> MFFQIEKVVLWSKEAKHKPRVIEFALNKVNLITGSSKSGKSSLIPIIDYCLGSSKCSIPVNTIRDTTAWYGVQIKTKHSRLLIARRDPSNQLSTSNAFFVEAENIEIPQNIEKHNVNIDTVKNRLNEISGVSNISFDFYDTGRIDKKRTSTRDLSAFNYQPQNIIANPNALFYKTDSFEHKSKLVTILPYVLGALSNTDIENQHRIKNLEEEYRKVERRLLKLKRQNEDWLSSAQAYVIKAMELGLVNSDKDIYQLKPERLLNVLKNIATKEIDYSTSAANIKYASEQEAEITKRSRDISNNLAKVKSRLQNINSMNRLANTHSDASRLKRERLSLSKWLLTQNDINSSLFSEPNEIRSLVLEPLARAFSNLEAELEVPIHVQGALSREKIYLEGELTRLASEMKDVNTQLKILRGNKRKLGYDAFSVGKFVGE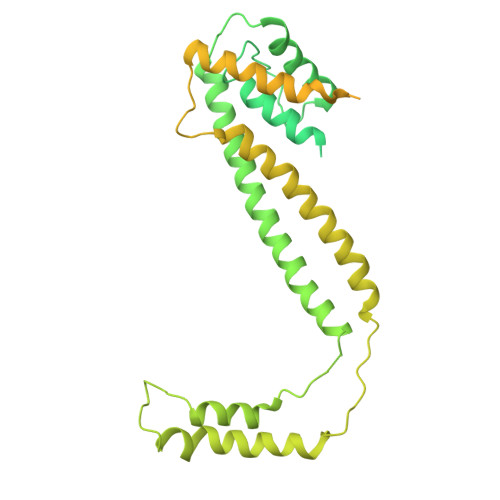VEKALSLMGESESESELSKEYKRLKKELSVLRLKIDPREFERKTKLQLAKVNKLASDWLPHLDTENPNAPISLHEKELTITVNSSGREDYLWEIGSGANWLSYHVAITLALHQHFSSLEASPVPNYIIYDQPSQVYFPSKLRHQATPEEDELALLEQDEDIVQVKKIFEAFNGAIEKTKDNLQIIVLDHAPSTLVKSIPKGHLVEEWRNGIKLIPLDWL> DKYQARELPLLKHGYSKKNMTAYNMFGFCCDNTPSGIFNIMDKKPT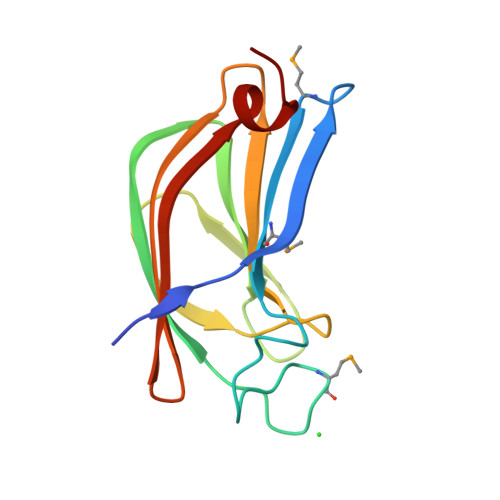EFLVNIYVGDNQGCKFIYAADTKGKQGEITQTGSFTAYLSGRNELLKLECKGKDSNIDYKVIAYANAIEYDRVGNLSYLVESGGL> TYPA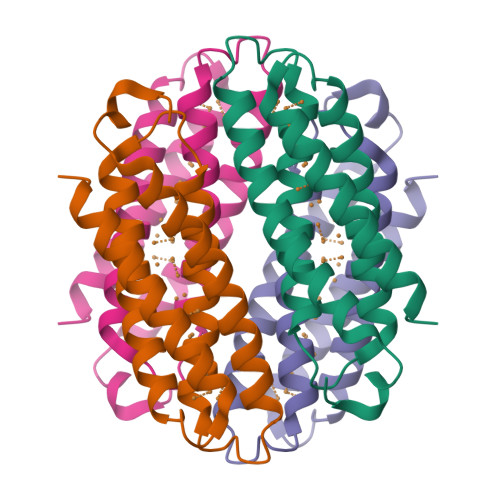DLGGVDREAMARCIEECLRCAQACTACADACLSEPTVADLTKCIRTDMDCADVCTATAAVLSRHTGYDANVTRAVLQACATVCAACGDECARHAGMHEACRVCAEACRSCEQACQELLAGLG> SDE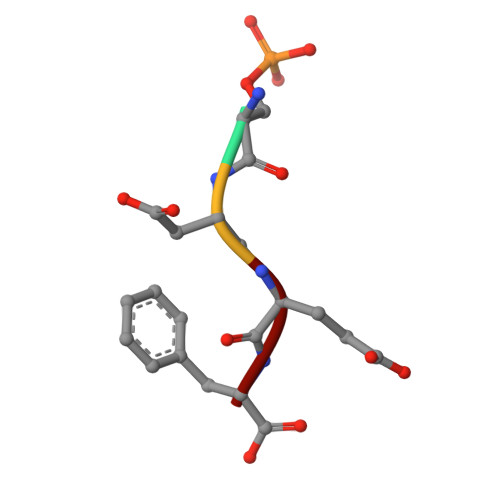F> MIKVEIKPSQAQFTTRSGVSRQG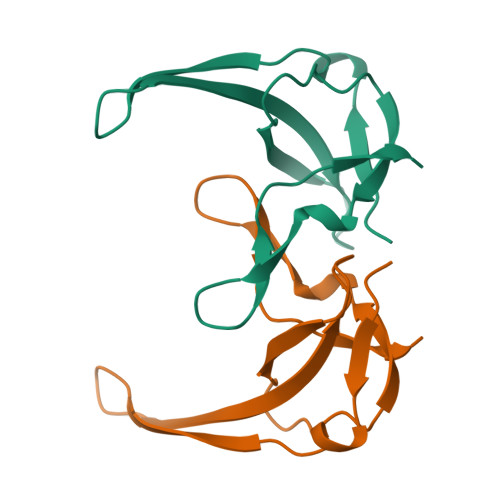KPYSLNEQLCYIDLGNEYPVLVKITLDEGQPAYAPGLYTVHLSSFKVGQFGSLMIDRLRLVPAK>[4x]MSRIVNVKLSLKRYEYEKPFHITGSVSSESRNVEVEIVLESGVKGYGEASPSFRVNGERVEALLAIEN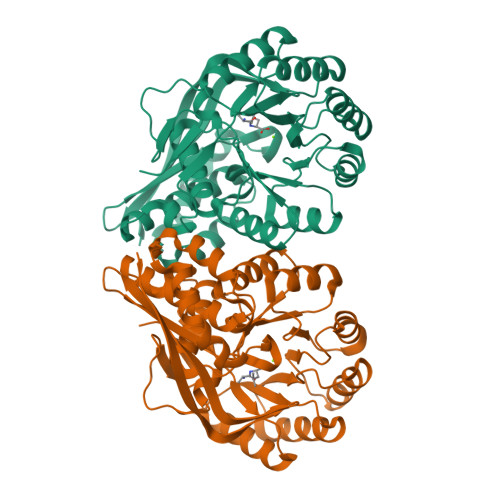AVREMITGIDVRNYARIFEITDRLFGFPSLKAAVQFATLDALSQELGTQVCYLLGGKRDEIETDKTVGIDTVENRVKEAKKIFEEGFRVIKIKVGENLKEDIEAVEEIAKVTRGAKYIVDANMGYTQKEAVEFARAVYQKGIDIAVYEQPVRREDIEGLKFVRFHSPFPVAADESARTKFDVMRLVKEEAVDYVNIKLMKSGISDALAIVEIAESSGLKLMIGCMGESSLGINQSVHFALGTGAFEFHDLDSHLMLKEEVFRGKFIQDGPRMRVKDQ> MVAASSRLMKELEEIRKAGMKNFRNIQVDEANLLTWQGLIVPDNPPYDKGAFRIEINFPAEYPFKPPKITFKTKIYHPNIDEKGQVCLPVISAENWKPA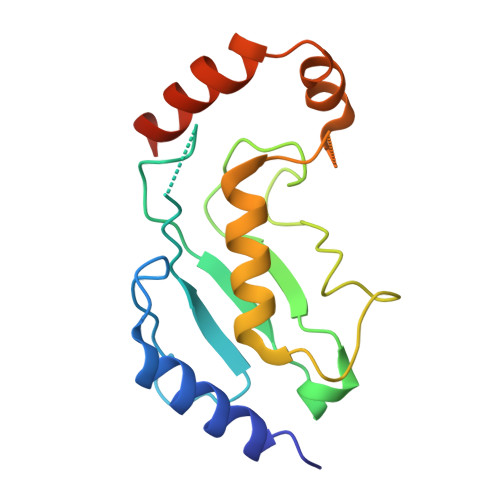TKTDQVIQSLIALVNDPQPEHPLRADLAEEYSKDRKKFAKNAEEFTKKYGEKRPVD2-[(1S)-1-cyclopropylethyl]-5-[4-methyl-2-[[6-(2-oxidanylidenepyrrolidin-1-yl)pyridin-2-yl]amino]-1,3-thiazol-5-yl]-7-methylsulfonyl-3H-isoindol-1-one | C27 H29 N5 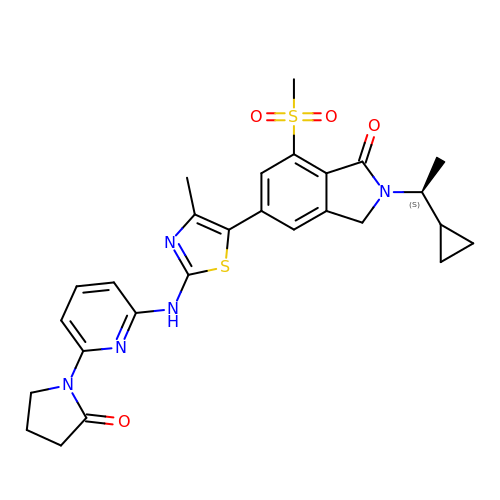O4 S2 | XOMFDZJQLSPGGV-INIZCTEOSA-N>MLAHSSSESPPESLPDAWTVLKTRTAVRNYAKEPVDDALIEQLLEAMLAAPTASNRQAWSFMVVRRPAAVRRLRAFSPGVLGTPAFFVVACVDRSLTDNLSPKLSQKIYDTSKLCVAMAVENLLLAAHAAGLGGCPVGSFRSDIVTSMLGIPEHIEPMLVVPIGRPATALVPSQRRAKNEVVNYESWGNRAAAPTA[2x];>[2x]MNPGETVLPPQLREEIALLAVYLLSSGRGLLEEPADYGIYRCTDGARRALQLLDEHGGSTARLTAVRERLDEVMFAPMGEDRDMGAILDDLCRQMADALPEIETP

Here, we report the structural characterization of the Streptomyces noursei enzyme AlbAB, a cyclodipeptide oxidase (CDO) carrying out α,β-dehydrogenations during the biosynthesis of the antibiotic albonoursin. We show that AlbAB is a megadalton heterooligomeric enzyme filament containing covalently bound flavin mononucleotide cofactors. We highlight that AlbAB filaments consist of alternating dimers of AlbA and AlbB and that enzyme activity is crucially dependent on filament formation.

3D helical reconstruction yielded a map with a global resolution of 3.14 Å where a single C2 symmetrical dimer of AlbA (AlbA2) and a single C2 symmetrical dimer of AlbB (AlbB2) form a heterotetramer representing the biologically relevant asymmetric unit of the filament. The AlbAB filament lacked rotational symmetry along the long axis, instead exhibiting repeating units of AlbA2 and AlbB2 with a helical rise of 46 Å per AlbA2 and AlbB2, a helical twist of 120°, a helical pitch of 138 Å, and an overall diameter of 100 Å. One FMN cofactor per AlbA monomer could be unambiguously localized in our cryo-EM density. Masked local refinement containing one AlbA2 and two surrounding AlbB2 units yielded an improved 2.78 Å map allowing confident model building for the dimers AlbA2 and AlbB2 as well as the bound FMN cofactors. The AlbA monomer consists of five α helices and four anti-parallel β strands. AlbA dimer formation is mediated by extensive interactions between helix α4 of both monomers, which is further stabilized by interactions with helix α1. AlbB forms a dimeric 8-helix bundle with each monomer containing four α helices arranged in an anti-parallel orientation similar to four-helix bundle proteins. The AlbB dimer is formed through extensive intermolecular interactions of 35 residues contained within helices α1, α2, and α4 in a knobs-into-holes packing scheme often found in four-helix bundle or coiled-coil proteins. The most significant inter-dimer interactions occur between helix α3 of AlbA and helices α1 and α2 of AlbB. The FMN binding site is located at the interface of the AlbA2 and AlbB2 dimers, with clearly visible cryo-EM density corresponding to an 8α-S-cysteinyl linkage between the side chain thiol of C115 of AlbA and the C8 carbon of FMN. The positively charged AlbA residues R24, R28, and R175 are highly conserved and coordinate the phosphate group of the FMN ribityl chain.3'-DEOXYADENOSINE | C10 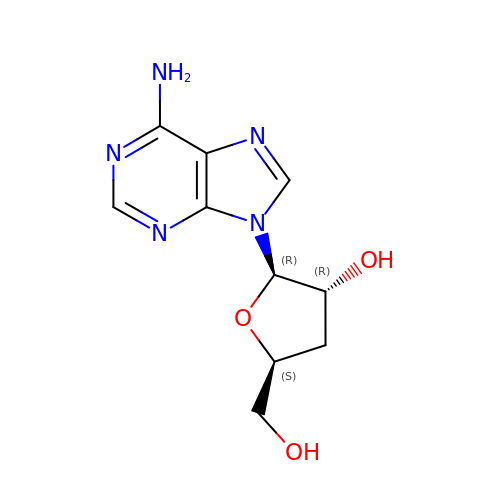H13 N5 O3 | OFEZSBMBBKLLBJ-BAJZRUMYSA-N> MIERGKFRSLTLVNWNGFFARTFDLDELVTTLSGGNGAGKSTTMAAFVTALIPDLTLLHFRNTTEAGATSGSRDKGLHGKLRAGVCYSTLDVINSRHQRVVVGVRLQQVAGRDRKVDIKPFMIQGLPTAIQPTQLLTENVGERQARVLPLNEL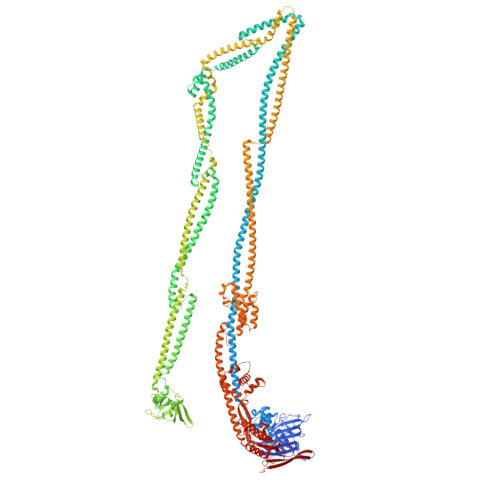KDRLDEMEGVQFKQFNSITDYHAQMFDLGVIPKRLRSASDRSKFYRLIEASLYGGISSAITRSLRDYLLPENSGVRKAFQDMEAALRENRITLEAIRVTQSDRDLFKHLITEATSYVSADYMRHANERRTHLDEALALRGELFGSHKQLATEQYRHVEMARELAEQSGASSDLETDHQAASDHLNLVQTAMRQQEKIDRYQVDLEELSYRLEEQTDVVEEAGELQAEYEARTEATEQEVDELKSQLADYQQALDVQQTRAIQYQQALQALERARELCRLPDLSVDNAEEWLETFQAKEQQATEALLALEQKLSVADAAHNQFEQAYQLVKNIVGETSRSEAWQSARELLRDWPSQRHLADRVQPLRMRLSELEQRLNNQQNAERLLSEFCKRQGRQYQAEDLEALQNELEARQEALSLSVNEGGERRMEMRQELEQLKQKIQSLTARAPVWLAAQDTLNQLCEQSGETLASSNDVTEYMQQLLEREREATVERDEVAAQKRELEKQIERLSQPSGAEDSRMIALAERFGGVLLSEIYDDITIDDAPYFSALYGPARHGIVVPDLSLVRPHLETLEDCPEDLYLIEGDPQSFDDSVFNAEEQTNAVLVKSSDRQWRYSRYPELPLFGRAARENRLEALNLERDALAERYATLSFDVQKIQRAHQAFSQFVGKHLSVAFDTDPEAEIRELRQRHTELEREVSRFEDQTQQQRQQYAQAKESLTTLNRLIPQVTLLLDETLIDRVEEVREEMDEAQEAARFLQQHGSALTKLEPMVAVLQSDPQQHEQLQQDYETAKHSQHQAKQQAFALVEIVQRRVHFSYSDSAGMLSENADLNDKLRQRLEHAESDRSRAREQLRQQQAQYSQFNQVLASLKSSYETKQDMLKELLQEMKDIGVQADANAEMRARERRDRLHEALSVNRSRVNQLEKQIAFCEAEMENVQKKLRKLERDYYQIREQVVSAKAGWCAVMRMVKDNGVERRLHRRELAYMEGGALRSMSDKALGALRLAVADNEHLRDALRLSEDPKRPERKVQFFIAVYQHLRERIRQDIIRTDDPVDAIEQMEIELARLTEELTAREQKLAISSKSVANIIRKTIQREQNRIRMLNQGLQAVSFGQVRGVRLNVNVRESHAILLDVLSEQQEQHQDLFNSQRLTFSEAMAKLYQRLNPQVDMGQRLPQTIGEELLDYRNYLELDVEVNRGSDGWLKAESGALSTGEAIGTGMSILVMVVQSWEEESRRLRGKDISPCRLLFLDQAARLDAKSIATLFELCERLQMQLIIAAPENISPEKGTTYKLVRKVFKNHEHVHVVGLRGFGQDAPATQLISDVTA>[6x]CGAATTA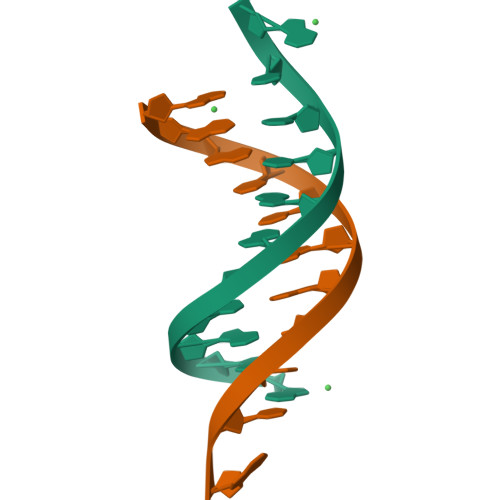ATTCG>VNVNFRCDNGVTQMGDSVYAVGNVSQLGNWSPASAVRLTDTSSYPTWKGSIALPDGQNVEWKCLIRNEADATLVRQWQSGGNNQVQAAAGAS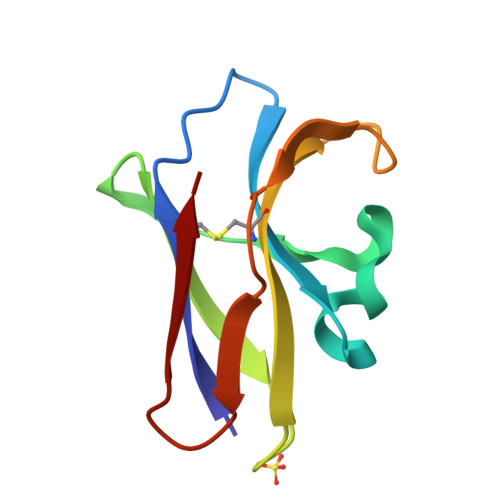TSGSF[2x]> GRSRLLEDFRNNRYPNLQLREIAGHIMEFSQDQHGSRFIQLKLERATPAERQLVFNEILQAAYQLMVDVFGNYVIQKFFEFGSLEQKLALAERIRGHVLSLALQMYGCRVIQKALEFIPSDQQNEMVRELDGHVLKCVKDQNGNHVVQKCIECVQPQSLQFIIDAFKGQVFALSTHPYGCRVIQRILEHCLPDQTLPILEELHQHTEQLVQDQYGNYVIQHVLEHGRPEDKSKIVAEIRGNVLVLSQHKFASNVVEKCVTHASRTERAVLIDEVCTMNDGPHSALYTMMKDQYANYVVQKMIDVA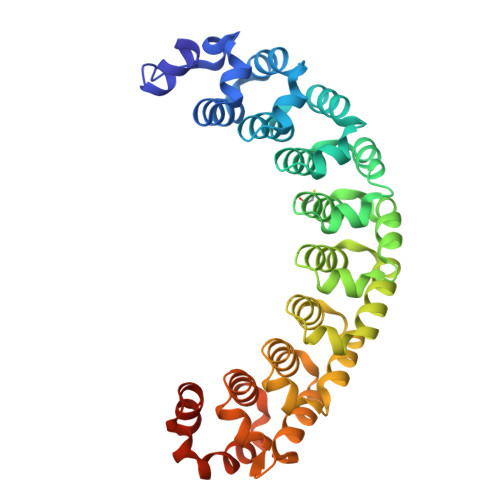EPGQRKIVMHKIRPHIATLRKYTYGKHILAKLEKYYMKNGVDLG>[2x]EAPHLVQVDAARALWPLRRFWRSTGFCPPLPHSQADPYVLSWDQQLNLAYVGAVPHRGIKQVRTHWLLELVTTRGSTGQ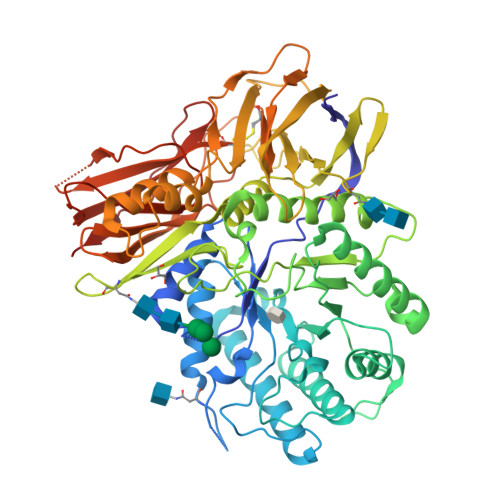GLSYNFTHLDGYLDLLRENQLLPGFELMGSASGHFTDFEDKQQVFEWKDLVSSLARRYIGRYGLAHVSKWNFETWNEPDHHDFDNVSMTMQGFLNYYDACSEGLRAASPALRLGGPGDSFHTPPRSPLSWGLLRHCHDGTNFFTGEAGVRLDYISLHRKGARSSISILEQEKVVAQQIRQLFPKFADTPIYNDEADPLVGWSLPQPWRADVTYAAMVVKVIAQHQNLLLANTTSAFPYALLSNDNAFLSYHPHPFAQRTLTARFQVNNTRPPHVQLLRKPVLTAMGLLALLDEEQLWAEVSQAGTVLDSNHTVGVLASAHRPQGPADAWRAAVLIYASDDTRAHPNRSVAVTLRLRGVPPGPGLVYVTRYLDNGLCSPDGEWRRLGRPVFPTAEQFRRMRAAEDPVAAAPRPLPAGGRLTLRPALRLPSLLLVHVCARPEKPPGQVTRLRALPLTQGQLVLVWSDEHVGSKCLWTYEIQFSQDGKAYTPVSRKPSTFNLFVFSPDTGAVSGSYRVRALDYWARPGPFSDPVPYLEVPVPRGPPSPGNP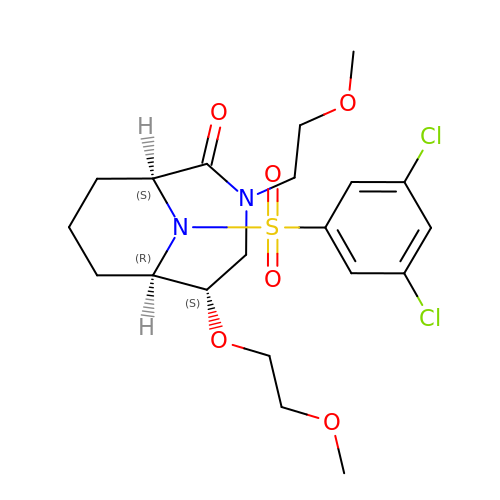(1S,5S,6R)-10-[(3,5-dichlorophenyl)sulfonyl]-5-(2-methoxyethoxy)-3-(2-methoxyethyl)-3,10-diazabicyclo[4.3.1]decan-2-one | C20 H28 Cl2 N2 O6 S | NVEGGBQTNWZDFS-QYZOEREBSA-N> MRDNQDLLVKRLGRLVNVLESKEFGGTTTVDKDLDVTKNVTRTDEPNEDNTPDYFSTGKDRVLVPDTEEWERLGFGIVAKTVNVR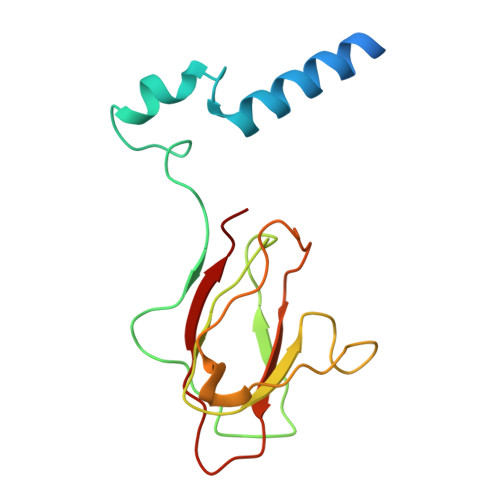TTDDVLLAFANPNTNGPTFKIRSNESPFTIGGDAGIDTAFMWLKKAESAQNDPAVEIIAYR> ASMTGNECPELQPPVHGKIEPSQAKYFFKDQVLVSCDTGYKVLKDNVEMDTFQIECLKDGTWSNKIPTCKIVDCRAPGELEHGLITFSTRNNLTTYKSEIKYSCQEPYYKMLNNNTGIYTCSAQGVWMNKVLGRSLPTCLPVCGLPKFSRKLMAR;> IFNGRPAQKGTTPWIAMLSHLNGQPFCGGSLLGSSWIVTAAHCLHQSLDPKDPTLRDSDLLSPSDFKIILGKHWRLRSDENEQHLGVKHTTLHPQYDPNTFENDVALVELLESPVLNAFVMPICLPEGPQQEGAMVIVSGWGKQFLQRFPETLMEIEIPIVDHSTCQKAYAPLK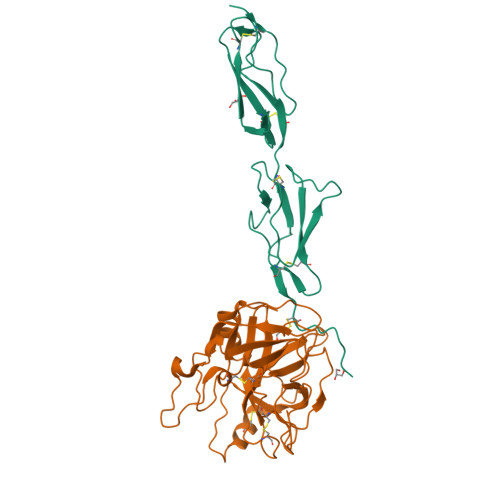KKVTRDMICAGEKEGGKDACAGDSGGPMVTLNRERGQWYLVGTVSWGDDCGKKDRYGVYSYIHHNKDWIQRVTGVRN>MTNLKPYIIYDWKETILKNSKDNYSINESIPKIFSKKICGGRFFNSTLSGNWKSWTLTDEGEGPHPVLKCTIDNGYLEIYSNTSSEKHSLKDIEIKVCMSIKPNSDGTHSLCKNSFYIKTNSLKLSEDRLILSHCLDKLILAWFKDNHKYIELFINRSRIQTRVEGDLSLLGWDIESSVSYKTMNEFIKKDNLYEKKFHQYMEVRRNEYTIDGEFGPWQMTTGADGQNIRFLCPIKSATYKINDDVYIAKPDNFIIIQVDLKYFDSKTTIIDPSGLNNGQQFNLKVKTDSTDEINAVILVGSRITDVNEDLYPGDDVSLEIVFKTWFNANIQKFTQIFSYILLNETSKIPEYQWLKPTQISYGSASVTMPDPSNPNKELSNLDASTFAAMAMVENHKNDRPNHAVDNRFLELSKTPAAFAISMPEFLKHFLVTGLQAMQIDNLDAFEVSSENLVITNKKKINFGKIQDQNRQVDALIEPNNFKLAIQNNQVVVEIVDATWQQVVGVTGHFGYRQAYNLILKNENNVYKPMLEESGDVTISYMVTEEAWKTTQDAIISATVGLVVGTIIGTAFSKLSDKLYKFLKSKFIVKNKKASLKISGKDINEVIEMSDISKPQLLSIKKANAKISTEEVGLISQNGSTSLENLAIFKNKPRPIGERVQILGLKLVSGLITTFGWSIGFVLPD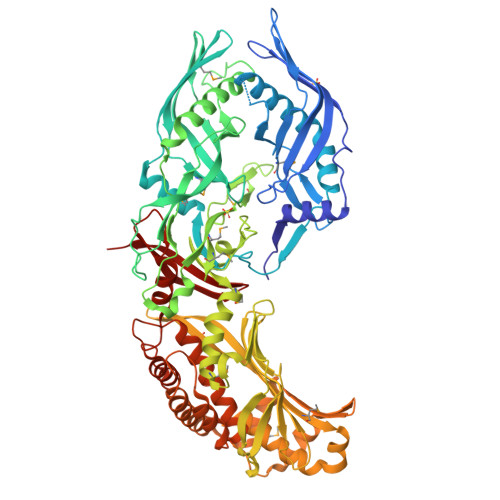ILKDVINANINNNFEVLPGIQQFTQQCIGSIQWPDNSELKIDFAKLQGVYLLGGNLVKIPESN[2x]N-acetylmannosamine-6-phosphate | C8 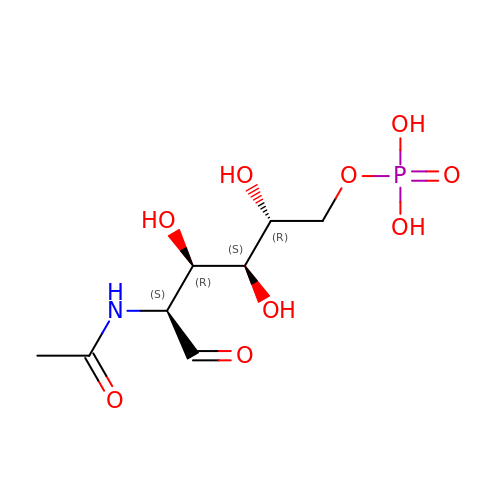H16 N O9 P | QDSLHWJDSQGPEE-WCTZXXKLSA-N PYRROLE-2-CARBOXYLATE | C5 H4 N O2 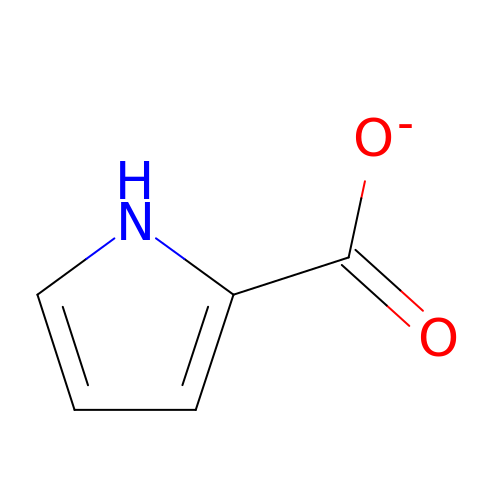| WRHZVMBBRYBTKZ-UHFFFAOYSA-M> AQVINTFDGVADYLQTYHKLPDNYITKSEAQALGWVASKGNLA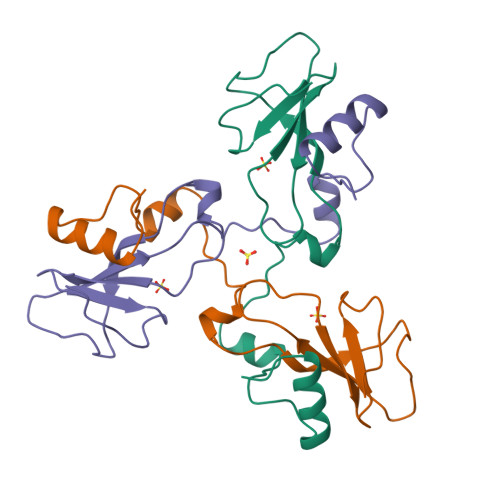DVAPGKSIGGDIFSNREGKLPGKSGRTWREADINYTSGFRNSDRILYSSDWLIYKTTDHYQTFTKIR> 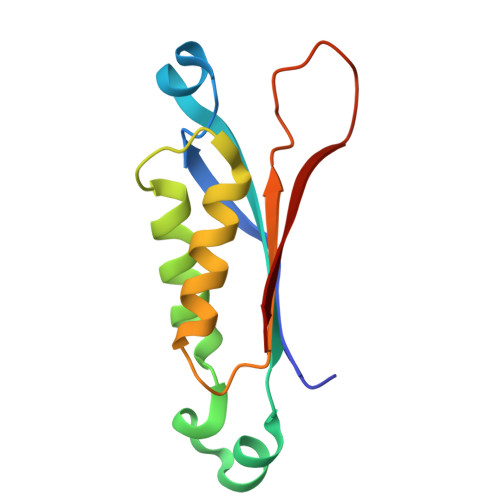MADRIELRGLTVHGRHGVYAHERVAGQRFVIDVTVWIDLAEAANSDDLADTYDYVRLASRAAEIVAGPPRKLIETVGAEIADHVMDDQRVHAVEVAVHKPQAPIPQTFDDVAVVIRRSR>GQKKSIYVAYTGGTIGMQRSDNGYIPVSGHLQRQLALMPEFHRPEMPDFTIHEYAPLIDSSDMTPEDWQHIANDIQQNYDLYDGFVILHGTDTMAFTASALSFMLENLAKPVIITGSQIPLAEDASDGQTNLLNALYLAANHPVNEVSLFFNNQLFRGNRT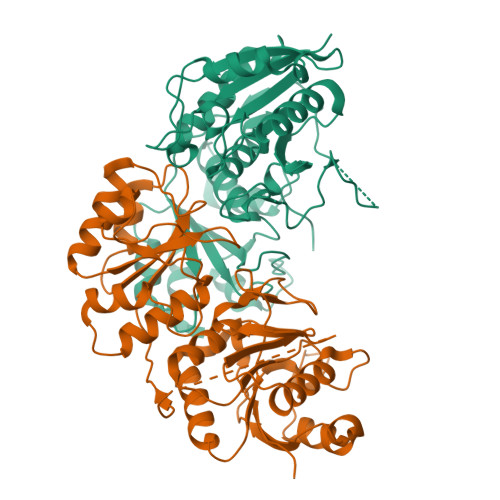TKAHADGFDAFASPNLSVLLEAGIHIRRQSSVVSPTSNGPLIVHRITPQPIGVVTIYPGISGAVVRNFLLQPVKALILRSYGVGNAPQKAELLDELKNASDRGIVVVNLTQSISGSVNMGGYATGNALAQAGVISGFDMTVEAALTKLHYLLSQSLSPNEIRQLMQQNLRGELTDTQ[4x]> GPGSDDEINAQSVWSEEISSNYPLCIKNLMEGLKKNHHLRYYGRQQLSLFLKGIGLSADEALKFWSEAFTRNGNMTMEKFNKELRYSFRHNYGLEGNRINYKPWDCHTILSKPRPGRGDYHGCPFRDWSHERLSAELRSMKLTQAQIISVLDSCQKGEYTIACTKVF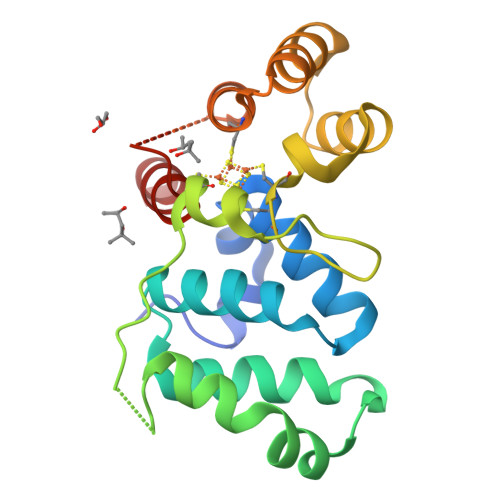EMTHNSASADLEIGEQTHIAHPNLYFERSRQLQK>SVKEVLFMNTGEGESSYVQNSSFTEKVASMAMPALENAVETLFSKDFHLFQAINAADLGCATGPNTFAVISTIKRMMEKKCRELNCQTLELQVYMNDLFGNDFNTLFKGLSSKVIGNKCEEVSCYVMGVPGSFHGRLFPRNSLHLVHSSYSVHWLTQAPKGLTSREGLALNKGRIYISKTSPPVVREAYLSQFHEDFTMFLNARSQEVVPNGCMVLILRGRQSSDPSDMQSCFIWELLAIAIAELVSQGLIDEDKLDTFNIPCYFPSLEEVKDIVERDGSFTIDHMEGFELDSLQMQENDKWVRGEKFAKIVRAFTEPIISNQFGHEIMDKLYDKFTHIVVSDL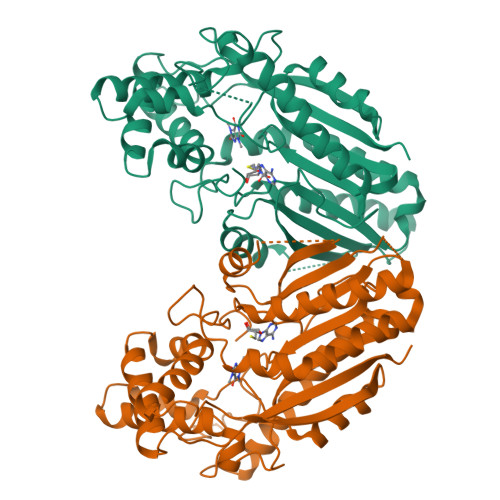EAKLPKTTSIILVLSKIVG[8x]>[4x]GIDPFTMNQLIQAQKKLLPDLLLVMQKRFEILQYIRLTEPIGRRSLSASLGISERVLRGEVQFLKEQNLVDIKTNGMTLTEEGYELLSVLEDTMKDVLGLTLLEKTLKERLNLKDAIIVSGDSDQSPWVKKEMGRAAVACMKKRFSGKNIVAVTGGTTIEAVAEMMTPDSKNRELLFVPARGGLGEDVKNQANTICAHMAEKASGTYRLLFVPGQLSQGAYSSIIEEPSVKEVLNTIKSASMLVHGIGEAKTMAQRRNTPLEDLKKIDDNDAVTEAFGYYFNADGEVVHKVHSVGMQLDDIDAIPDIIAVAGGSSKAEAIEAYFKKPRNTVLVTDEGAAKKLLRDE

The SorC family of transcriptional regulators plays a crucial role in controlling the carbohydrate metabolism and quorum sensing. A typical SorC protein comprises an N-terminal DNA-binding domain (DBD) of a helix–turn–helix (HTH) motif, along with a C-terminal Rossmann-like fold effector-binding domain (EBD). SorC repressors generally form tetramers as they bind to their operators located in promoter regions of regulated genes.

CggR functions as a repressor of the hexacistronic gapA operon encoding CggR itself and five crucial enzymes involved in the triose phosphate interconversion during glycolysis. We determined the structure of CggR bound to the complete DNA operator, referred to here as OLR. The DNA duplex OLR contains the full-length operator sequence of 45 bp, located between positions +32 and +77 relative to the transcription start point of the gapA operon. Our 2D particle classification indicates that, when bound to DNA, CggR forms a tetrameric assembly with a global C2 symmetry. The C2 symmetry was clearly apparent also in the reconstructed map refined without enforcing any symmetry, and the final 3D reconstruction using 220146 particles was therefore refined with C2 symmetry to a resolution of 4.3 Å (statistics in Table 2). Each monomer of CggR contains an N-terminal two-β-stranded wHTH motif with an extension of a C-terminal helix followed by a C-terminal effector-binding domain that shares great homology with other members of the SorC family. The dimerization is mediated through DNA-binding domains, predominantly through a swap of the N-terminal α1 helices. Two CggR dimers come together to form a tetrameric assembly via an interaction between the EBDs of the two neighboring dimers. The interaction of CggR with DNA is mediated by DBD dimers, each interacting with one half-operator, wedging into two consecutive major grooves. The conformation of the operator DNA is significantly affected by CggR binding and exhibits a profound bend in the regions contacted by DBD dimers. Another noteworthy feature of the bound DNA is the apparent kink in the middle of the DNA duplex, where the central minor groove, flanked by the DBD dimers, is substantially widened.4-chloranyl-2-[[5-chloranyl-2-(5-methoxy-1,3-dihydroisoindol-2-yl)-1,3-thiazol-4-yl]carbonyl-methyl-amino]-5-fluoranyl-benzoic acid | C21 H16 Cl2 F N3 O4 S | 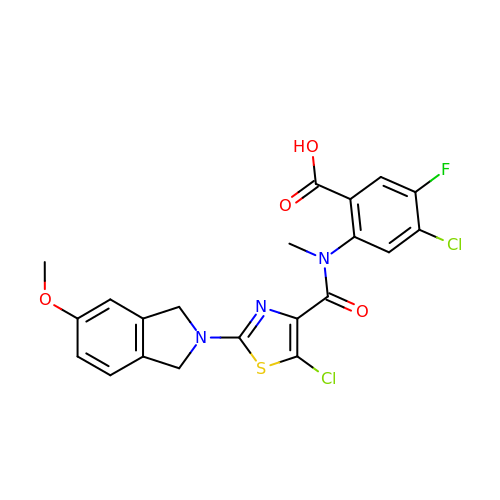LTJYYDAAQPZAGJ-UHFFFAOYSA-N> SLQDPCSNCPAGTFCDNNRNQICSPCPPNSFSSAGGQRTCDICRQCKGVFRTRKECSSTSNAECDCTPGFHCL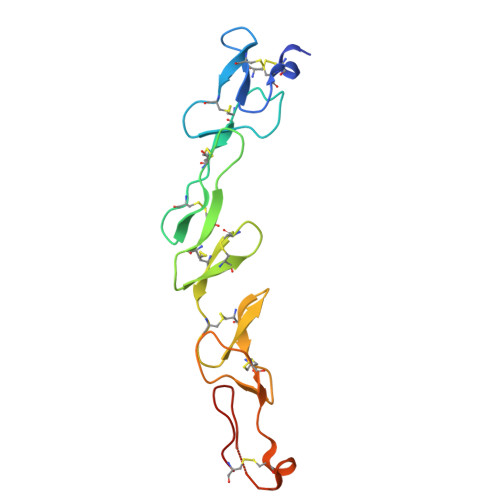GAGCSMCEQDCKQGQELTKKGCKDCSFGTFNDQKRGICRPWTNCSLDGKSVLVNGTKERDVVCGP>MTTQAPTFTQPLQSVVVLEGSTATFEAHISGFP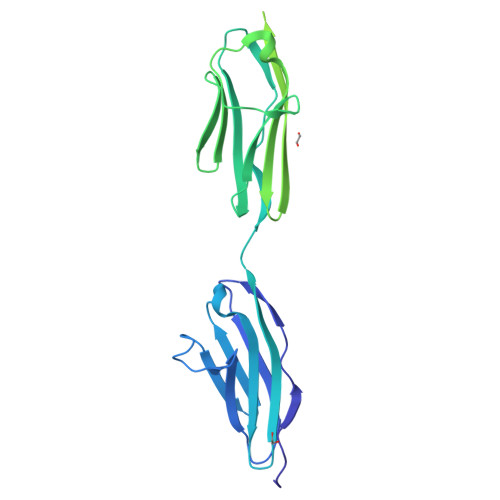VPEVSWFRDGQVISTSTLPGVQISFSDGRAKLTIPAVTKANSGRYSLKATNGSGQATSTAELLVKAETAPPNFVQRLQSMTVRQGSQVRLQVRVTGIPTPVVKFYRDGAEIQSSLDFQISQEGDLYSLLIAEAYPEDSGTYSVNATNSVGRATSTAELLVQGETTQAPTFTQPLQSVVVLEGSTATFEAHISGFPVPEVSWFRDGQVISSGRGDSSPGVQISFSDGRAKLTIPAVTKANSGRYSLKATNGSGQATSTAELLVKAETAPPNFVQRLQSMTVRQGSQVRLQVRVTGIPTPVVKFYRDGAEIQSSLDFQISQEGDLYSLLIAEAYPEDSGTYSVNATNSVGRATSTAELLVQGE[2x]> MAWPKVQPEVNIGVVGHVDFGKTTLVQAITGIWTSKHSEELKRGMTIKLGYAETNIGVCESCKKPEAYVTEPSCKSCGSDDEPKFLRRISFIDAPGHEVLMATMLSGAALMDGAILVVAANEPFPQPQTREHFVALGIIGVKNLIIVQNKVDVVSKEEALSQYRQIKQFTKGTWAENVPIIPVSALHKINIDSLIEGIEEYIKTPYRDLSQKPVMLVIRSFDVNKPGTQFNELKGGVIGGSIIQGLFKVDQEIK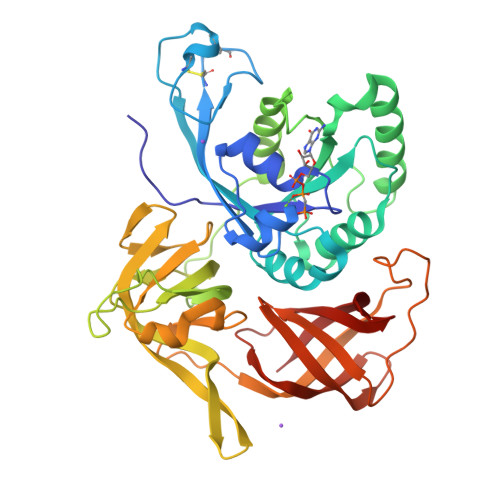VLPGLRVEKQGKVSYEPIFTKISSIRFGDEEFKEAKPGGLVAIGTYLDPSLTKADNLLGSIITLADAEVPVLWNIRIKYNLLERVVGAKEMLKVDPIRAKETLMLSVGSSTTLGIVTSVKKDEIEVELRRPVAVWSNNIRTVISRQIAGRWRMIGWGLVEI> GMTEQQLREEMVQIGASLFSRGYATGSAGNLSLLLPDGNLL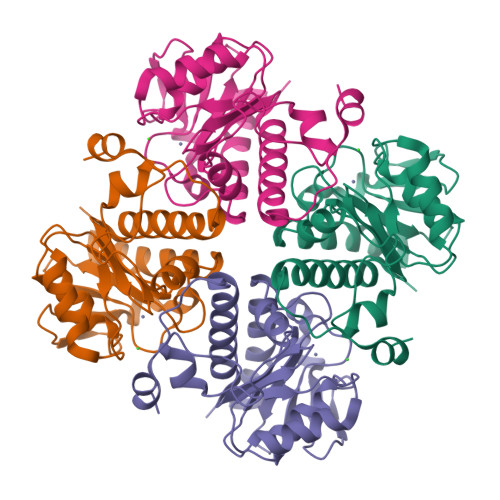ATPTGACLGELQAQRLSVVTLQGEWISGDKPSKEVTFHRAVYLHNPACKAIVHLHSHYLTALSCLQGLDPHNCIRPFTPYVVMRVGDVPVVPYYRPGDDRIAQALAGLAPRYNAFLLANHGPVVTGSSLREATNNTEELEETARLIFTLGNREIRYLTADEVKELR>[2x]SGSSLQQHLSNRDPRPLRDKNFQSAIQEEIYDYLKKNKFDIETNHPISIKFLKQPTQKGFIIIFKWLYLRLDPGYGFTKSIENEIYQILKNLRYPFLESINKSQISAVGGSNWHKFLGMLHWMVRTNIKLDMCLNKVDRSLINQNTQEITILSQPLKTLDEQDQRQERYELMVEKLLIDYFTESYKSFLKLEDNYEPSMQELKLGFEKFVHIINTDVTSTELKLEELKVDLNRKRYKLHQQVIHVIDITSKFKINIQSSLENSENELGNVIEELRNLEFETEHNVTN;>MKLRRKSILHTIRNSIASGARISLGSGAARVVNGPVSRNQDVFPILDLQELVICLQSCDFALATQENISRPTSDYMVTLYKQIIENFMGISVESLLNSSNQETGDGHLQEENENIYLDTLNVLVLNKICFKFFENIGVQDFNMTDLYKPEAQRTQRLLSAVVNYARFREERMFDCNSFILQMESLLGQINKLNDEIKQLQKDFEVEVKEIEIEYSLLSGHINKYMNEMLEYMQ[2x]

The bridge between centromere-associated kinetochore assemblies and spindle microtubules is the Ndc80 complex (Ndc80c), a heterotetramer, conserved from yeast to mammals, with globular elements at both ends of an approximately 600 Å long, largely α-helical coiled-coil shaft. Closely paired calponin homology (CH) domains of Ndc80 and Nuf2 at one end, augmented by a flexible, N-terminal extension of Ndc80, form a microtubule-attachment module. The coiled-coil shaft of Ndc80 : Nuf2 has two specializations—a kink or hinge at about 160 Å from the globular end and a so-called ‘loop’ at about 240 Å. At least three interactions involve subunits of the DASH/Dam1 complex (Dam1c, consisting of Ask1, Dad1, Dad2, Dad3, Dad4, Dam1, Duo1, Hsk3, Spc19 and Spc34), which coordinates end-on attachment of multiple Ndc80c rods around the splayed plus end of a kinetochore microtubule.

The predicted structure of the docked segment suggested that a fusion construct of part of the Dam1 C terminus (residues 252–305) with the Nuf2 N terminus, combined with a deletion of residues between the two conserved stretches (residues 271–289), might ensure high local concentration and increase the likelihood of obtaining informative crystals. We therefore made the inferred Ndc80 : Dam1-Nuf2 fusion construct as part of the dwarf-Ndc80c, expressed and purified the recombinant protein, and obtained crystals in space group P3212 (a = b = 130.0 Å, c = 216.3 Å). The Spc24-Scp25 component had dissociated during crystallization, and only the Ndc80 : Dam1-Nuf2 heterodimer was present in the crystals. Dam1 binds Ndc80 : Nuf2 with an α-helical segment, which rests in a cleft between the coiled-coil and the globular head domains, and an extended segment, which runs along the N terminus of Nuf2, but also contacts Ndc80. A salt bridge between Dam1 Arg299 and Ndc80 Asp295, both conserved across budding yeasts, anchors the C-terminal extended segment of the Dam1 fragment. The Dam1 sequence in the structure also includes three serines (residues 257, 265 and 292), the first and third conserved among budding yeasts and the second largely so, that are potential Ipl1 targets for regulating Ndc80c binding. The structure suggests that phosphorylation of serines 257 and 265 would substantially weaken the contact. The side chain of Ser257 is close to conserved Ndc80 glutamate 276 and its phosphorylation would result in electrostatic repulsion. We observed that density for the Dam1 segment fused to the second copy of the Ndc80 : Nuf2 head in the asymmetric unit was much weaker than the first, and its appearance was of insufficient clarity to build a molecular model. Thus, the crystal packing prevented uniform ordering of the Dam1 segment at position 2.>HPEFLKAGKEPGLQIWRVEKFDLVPVPTNLYGDFF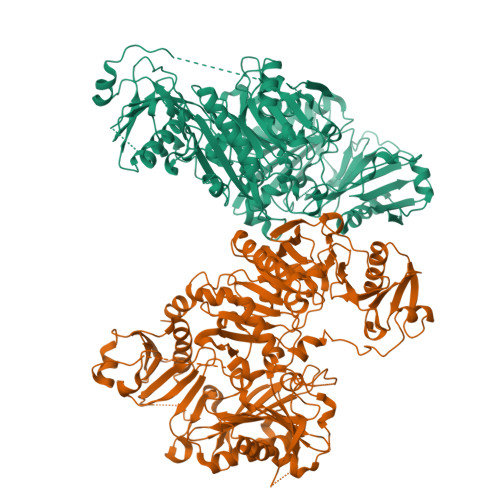TGDAYVILKTVQLRNGNLQYDLHYWLGNECSQDESGAAAIFTVQLDDYLNGRAVQHREVQGFESATFLGYFKSGLKYKKGGVASGFKHVVPNEVVVQRLFQVKGRRVVRATEVPVSWESFNNGYCFILDLGNNIHQWCGSNSNRYERLKATQVSKGIRDNERSGRARVHVSEEGTEPEAMLQVLGPKPALPAGTEDTAKEDAANRKLAKLYKVSNGAGTMSVSLVADENPFAQGALKSEDCFILDHGKDGKIFVWKGKQANTEERKAALKTASDFITKMDYPKQTQVSVLPEGGETPLFKQFFKNWRDPDQTDGLGLSYLSSHIANVERVPFDAATLHTSTAMAAQHGMDDDGTGQKQIWRIEGSNKVPVDPATYGQFYGGDSYIILYNYRHGGRQGQIIYNWQGAQSTQDEVAASAILTAQLDEELGGTPVQSRVVQGKEPAHLMSLFGGKPMIIYKGGTSREGGQTAPASTRLFQVRANSAGATRAVEVLPKAGALNSNDAFVLKTPSAAYLWVGTGASEAEKTGAQELLRVLRAQPVQVAEGSEPDGFWEALGGKAAYRTSPRLKDKKMDAHPPRLFACSNKIGRFVIEEVPGELMQEDLATDDVMLLDTWDQVFVWVGKDSQEEEKTEALTSAKRYIETDPANRDRRTPITVVKQGFEPPSFVGWFLGWDDDYWSVDPLDRAMAELAA[2x]> MDGSGEQPRGGGPTSSEQIMKTGALLLQGFIQDRAGRMGGEAPELALDPVPQDASTKKLSESLKRIGDELDSNMELQRMIAAVDTDSPREVFFRVAADMFSDGNFNWGRVVALFYFASKLVLKALSTKVPELIRTIMGWTLDFLRERLLGWIQDQGGWDGLLSYFGSS;> DMRPEIWIAQELRRIGDEFNAYYARR

The intrinsic pathway to apoptosis is regulated by interactions between members of three factions of the Bcl-2 protein family: the BH3-only proteins such as Bim and Bid, which initiate the process, the essential effectors Bax and Bak, and the prosurvival members, which oppose the action of both other factions. Unlike Bak, which is constitutively anchored in the mitochondrial outer membrane (MOM) via its C-terminal segment, Bax is largely cytosolic in healthy cells and accumulates at the MOM only upon a death signal. Core/latch dimers of Bax and Bak form on treatment of the monomeric proteins with certain BH3 peptides and CHAPS, and Bax and Bak core domains form symmetric homodimers, supporting that unlatching the core domain is a necessary step to Bax and Bak oligomerisation and permeabilisation of the MOM. Bim and Bid are both potent direct activators of Bax, but Bim is less dependent on interactions via its ‘h0' residues than is Bid.

Here we describe the crystal structures of BimBH3 26- and 20-mer peptides bound to BaxΔC26. We therefore made a complex instead with a BaxΔC26 construct, this crystallised in different conditions to those used for the BidBH3:BaxΔC21 complex. The C terminus of BaxΔC26 (G166) is visible together with one residue from the vector (serine), whereas the C-terminal residues 168–171 of BaxΔC21 in the BidBH3 complex are disordered. The BimBH3 peptide is helical until residue Y163, as previously observed in complexes of BimBH3 with prosurvival molecules. The Bim and Bid peptides differ in length, but the structures of the helical segments from residues ‘h0'–‘h4' are in close alignment. The C-terminal residues of the Bim peptide (–R–R– Figure 1a) are disordered. The first of the ‘h0' residues of BimBH3, P144, makes similar hydrophobic contacts with Bax as its counterpart I82 in BidBH3. The alkyl moiety of BimBH3 residue E145 occupies the same space as the BidBH3 residue I83, but its carboxylate moiety does not form a typical pair of hydrogen bonds with the guanidinium of Bax R94. In the BimBH3 complex structure, Bim R153 forms a planar stack, with the interactions network formed by Bim D157, Bax R109 and Bax D102. Bim R153 is also hydrogen bonded with Bax S101 and the backbone carbonyl groups of Bax D97 and M98. A small shift in the position of Bax helix α3 between the two structures may be because of the contacts between Bim W147 and Bax M79.>[3x]GSKKWFSEFSIMWPGQAFSLKIKKILYETKSKYQNVLVFESTTYGKVLVLDGVIQLTEKDEFAYHEMMTHVPMTVSKEPKNVLVVGGGDGGIIRELCKYKSVENIDICEIDETVIEVSKIYFKNISCGYEDKRVNVFIEDASKFLENVTNTYDVIIVDSSDPIGPAETLFNQNFYEKIYNALKPNGYCVAQCESLWIHVGTIKNMIGYAKKLFKKVEYANISIPTYPCGCIGILCCSKTDTGLTKPNKKLESKEFADLKYYNYENHSAAFKLPAFLLKEIENI

Spermidine synthase (SpdS; putrescine aminopropyltransferase) catalyzes the transfer of the aminopropyl moiety from decarboxylated S-adenosylmethionine to putrescine, leading to the formation of spermidine and 5′-methylthio­adenosine (MTA). In this work, X-ray crystallography was used to examine ligand complexes of SpdS from the malaria parasite Plasmodium falciparum (PfSpdS). The active site of SpdS is located between the domains and consists of two interconnected clefts for binding dcAdoMet and putrescine. A conserved flexible structural element called the gatekeeper loop covers the active site of the enzyme.

In contrast to the other inhibitors tested, the complex with BIPA was obtained without any ligand bound to the dcAdoMet-binding site of the enzyme. In the structure containing only BIPA, electron density for the ligand was detected in the active sites of chains A and C but not chain B, presumably owing to crystal contacts with the neighbouring asymmetric unit restricting the conformation of the monomer. In addition, the gatekeeper loop in chain B was disordered and could not be built into electron density. Despite the different scaffold, the benzimidazole moiety of BIPA occupies the binding site of the dcAdoMet aminopropyl group. Although BIPA has no inhibitory activity at 1 mM (unpublished data), it is unique among the ligands studied to date in crystallizing with PfSpdS when bound alone, despite anchoring only the N-terminal part of the gatekeeper loop. The remaining part of the loop has a conformation similar to that found in structures with ligands bound to both parts of the active site. On the other hand, the complex with BIPA shows that ligands with certain scaffolds may bind alone to the enzyme and still form the interactions required for loop stabilization. The binding mode of BIPA, on the other hand, enables a different manner of loop stabilization. Thus, one amino group of the imidazole ring appears to stabilize the N-terminal part of the gatekeeper loop by forming a hydrogen bond to Asp196, although the backbone carbonyls of Ser197 and Ser198 and the side chain of Ser198 are also at a hydrogen-bonding distance. The absence of interactions with Pro203 at the other end of the loop may be one of the reasons that BIPA is a poor inhibitor of SpdS.Enhanced ABA levels elicited in response to drought are perceived by the PYR/PYL/RCAR family of ABA receptors and the clade A subfamily of protein phosphatases type 2C (PP2Cs), which act as necessary ABA co-receptors in ternary complexes. In the resting state, PYLR/PYL/RCAR receptors display an open ABA binding cavity flanked by two highly conserved loops, named as gate/CL2/β3-β4 loop and latch/CL3/β5-β6 loop. Specifically, both gate and latch loops define a surface that enables the receptor to dock into the PP2C active site. The formation of receptor-ABA-phosphatase complexes causes the dissociation of different PP2C-SnRK2 complexes and abolishes PP2C-mediated inhibition of the SnRK2s, triggering ABA response.

In contrast, a fourfold increase in the IC50 of ABA was determined in the synthetic receptor compared to its WT. The synthetic CsPYL15m receptor displays a similar chain of stabilizing interactions as AtPYL10 along the five mutated residues (left and middle). First, we selected a dimeric receptor and designed a series of mutations that increased its affinity for the synthetic ligand while reducing the affinity for ABA. Therefore, we did not observe constitutive activation of ABA signaling in vivo, which otherwise could be detrimental in the absence of stress.

> MNNNKAEADTSSSMADPETRPTYTTHHLAIPSGVTQDEFDELKQSVVEFHTYQLSQNQCSSLLAQRIRAPNDVVWSIVRRFDQPQTYKHFIKSCSVSDNFTMAVGSTRDVNLISGLPAATSTERLDILDDDRQVLGISIIGGEHRLRNYRSVISVHGFNRDGAICTVALESYVVDVPEGNTEEDTRLFADTVVKLNLQKLVSVAESQVI;> RSVYELDCIPLWGVVSIQGNRSEMEDAFAVSPHFLKLPIKMLMGDHEGMSPSLTHLTGHFFGVYDGHGGHKVADYCRDRLHFALAEEIERIKDELCKRNTGAGRQVQWDKVFTSCFLTVDGEIEGKIGRAVVGSSDKVLEAVASETVGSTAVVALVCSSHIVVSNCGDSRAVLFRGKEAMPLSVDHKPDREDEYARIENAGGKVIQWQGARVFGVLAMSRSIGDRYLKPYVIPEPEVTFMPRSREDECLILASDGLWDVMNNQEVCEIARRRILMWHKKNGAPPLAERGKGIDPACQAAADYLSMLALQKGSKDNISIIVIDLKAQRKFKTRT> QSHVDNPFVGASGYVNPDYSKEVDSSIVKVKDVQLKAKMQVVKSYPTYVWLDSIDAIYGGSRNAGRLSLQGHLNAALAQKKANTPITVGLVIYDMPGRDCHALASNGELPLTQAGLQRYKTEYIDVIASTLANPKYKGLRIVNIIEPDSLPNLVTNQSTPACGQASSSGIYEAGIKYALDKLHAIPNVYNY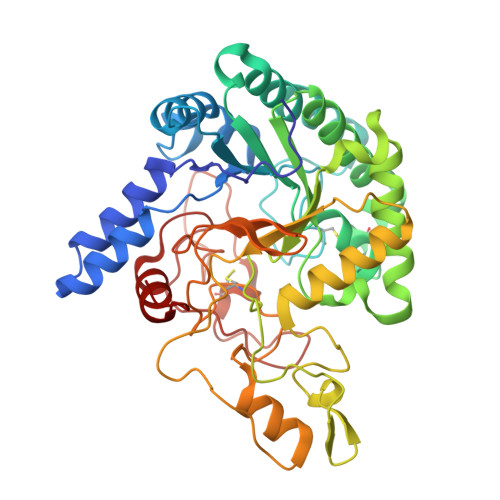MDIGHSGWLAWRSNMTPAISLYTRVVQGTAAGLASADGFITNTANYTPLHEPNLPNPDLTIGGQPISSSTFYQWNSVFDESTYAEVLYNAFVGAGWPSKIGFLIDTGRNGWGGSARPTSASGNDVNTYVNSGRVDRRLHRGNWCNQSGAGIGMPPTAAPGGHIHAYVWGKGGGESDGSSKYIPNKQGKGFDRYCDPTYTTPDGTLTGALPNAPIAGTWFHAHFVQLVTNAYPAI> A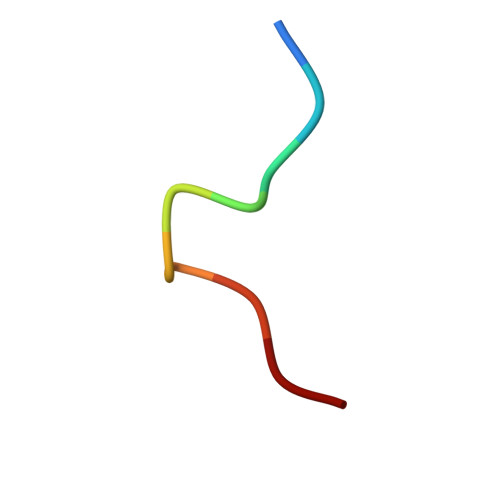GGPTIEEVD>SGKNPVESVSVEFEAKSARDGAWYDVAAFLSHRLFESGDPEVRVRFSGFGAEEDEWINVRKCVRQRSLPCEATECVAVLPGDLILCFQEGKDQALYYDAHVLDAQRRRHDVRGCRCRFLVRYDHDSSEEIVPLRKVCRRPETDYRLQILHAARAAATN[2x];> AR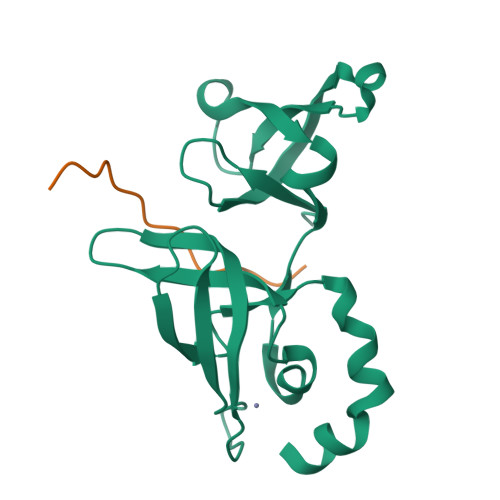TKQTARMSTGGKAPRKQ> MKKRKSSKVFKSTIAPEEKLRYIGNHKQAFDIEPLYPLALFEEFVATTGDCIIECSGKIKQDQLYPARIDLQFSDKHHFHNIHTSIDFLKRAASRTDVNLNLDILATFLAGNFDYSKVQNILAGIDLRQNLGESKLKLFIRIGDYPAKMAVAKHLCNITPESEAMLRSD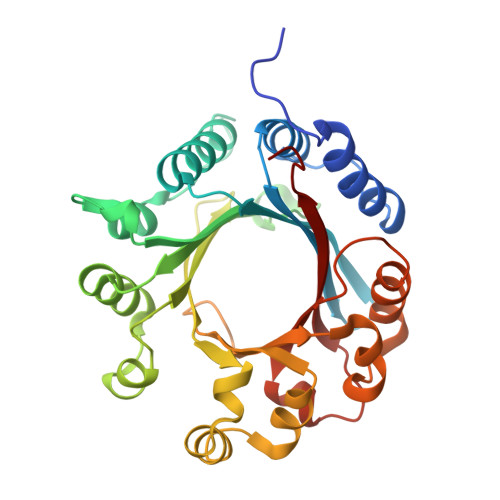TLHIGFDFYLDGRSAIELYPELKKDEFNHPFIYNQLKTILSPEALKPLPLCNLFGIGLSPANEANVLYYHLENIEDFLSYFPINDTARRVHDFYLQQEGSRRMWVALSESEMKAGRINNVNLYYSKAFTSQNP> MIERGKFRSLTLINWNGFFARTFDLDELVTTLSGGNGAGKSTTMAAFVTALIPDLTLLHFRNTTEAGATSGSRDKGLHGKLKAGVCYSMLDTINSRHQRVVVGVRLQQVAGRDRKVDIKPFAIQGLPMSVQPTQLVTETLNERQARVLPLNELKDKLEAMEGVQFKQFNSITD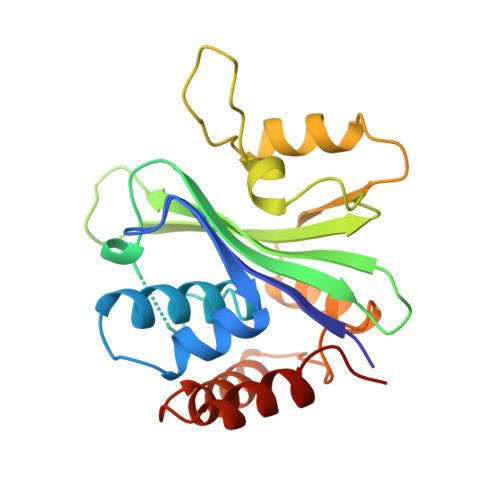YHSLMFDLGIIARRLRSASDRSKFYRLIEASLYGGISSAITRSLRDYLLPENSG> MSEKHPGPLVVEGKLTDAERMKHESNYLRGTIAEDLNDGLTGGFKGDNFLLIRFHGMYQQDDRDIRAERAEQKLEPRHAMLLRCRLPGGVITTKQWQAIDKFAGENTIYGSIRLTNRQTFQFHGILKKNVKPVHQMLHSVGLDALATAWDMNRNVLCTSNPYESQLHAEAYEWAKKISEHLLPRTRAYAEIWLDQEKVATTDEEPILGQTYLPRKFKTTVVIPPQNDIDLHANDMNFVAIAENGKLVGFNLLVGGGLSIEHGNKKTYARTASEFGYLPLEHTLAVAEAVVTTQRDWGNRTDRKNAKTKYTLERVGVETFKAEVERRAGIKFEPIRPYEFTGR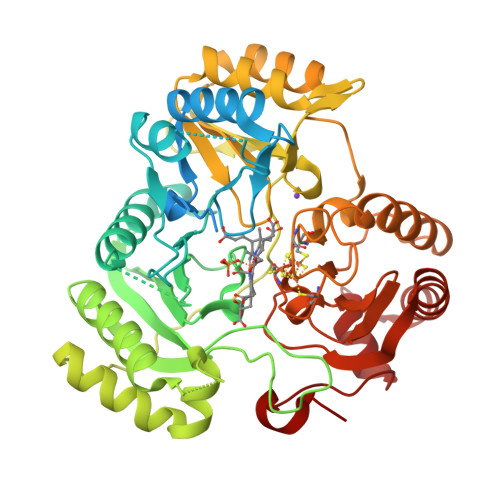GDRIGWVKGIDDNWHLTLFIENGRILDYPARPLKTGLLEIAKIHKGDFRITANQNLIIAGVPESEKAKIEKIAKESGLMNAVTPQRENSMACVSFPTCPLAMAEAERFLPSFIDNIDNLMAKHGVSDEHIVMRVTGCPNGCGRAMLAEVGLVGKAPGRYNLHLGGNRIGTRIPRMYKENITEPEILASLDELIGRWAKEREAGEGFGDFTVRAGIIRPVLDPARDLWD>[2x]MGQQRWITQAYLQRIEEGKKEWAQFAQEIKEGKRKSFVEHLEERGLIHDVVGDRDLLHRVFTEKRVGIYAGVDPTAPSMHVGHMLPFMVLAWGYVWGLPVTFLLGGATSRVGDPTGRLKGREQVHSSVRKAN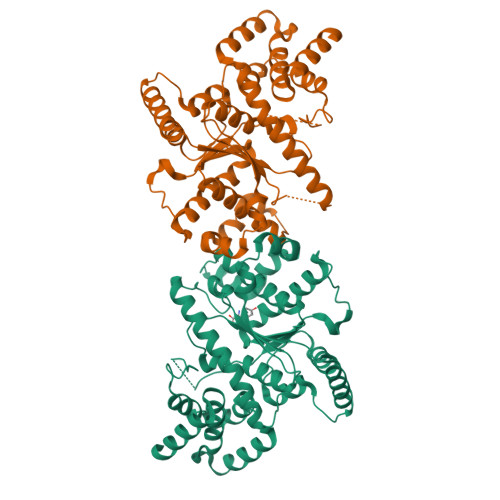MASMHMQLKKLGASIERYGEKHGYKRQMIWRRTLTNNNVWWNKTPLLEVLRDLGAYIRIGPMLGRDTVKNRMERGDGMSFAEFTYPLMQAWDWWMLFKNGCQVQVGGSDQYGNILFGVGAVKTISKNTVLQEDNNPLSDDLDKPIGFTTPLLTTSSGEKFGKSAGNAIWLDKDMTSTFELYQFFVRTPDDAVERYLKMFTFLPIPEISKIMEEQNQDPSRRVAQHALAYEFVELIHGKDEADAVSMQHRQLFRPRTSTAEPTP>[2x]MTLSIPPSIQCQTEAACRLITRVTGDTLRAIHLYGSAVAGGLKPNSDIDLLVTICQPLTEAQRATLMQELLALSSPPGASAEKRALQVTVVLYSQLVPWCFPPSREMQFGEWLREDICQGIYEPAQQDWDMVLLITQILETSIPLKGERAERLFTPAPAAQLLKALRYPLDLWQSTADVQGDEYHIVLTLARIWYTLSTGRFTSKDAAADWLLPQLPEDYAATLRAAQREYLGLEQQDWHILLPAVVRFVDFAKAHIPTQFTKGHHHHHH

Aminoglycoside (3″)(9) adenylyltransferase AadA from Salmonella enterica belongs to the ANT(3″)-Ia family and catalyzes the magnesium-dependent O-adenylation of streptomycin and spectinomycin at positions 3″ and 9, respectively. Modification of streptomycin and spectinomycin by O-phosphorylation or O-nucleotidylation prevents the drugs from binding to their respective binding sites on the ribosome (for reviews, see Refs. 9 and 10). In the apo state, AadA has a monomeric two-domain structure with the active site located between an N-terminal adenylyltransferase domain and a C-terminal helical domain. We here present crystal structures of wild type (WT) AadA with ATP or ATP and streptomycin and of an active-site mutant in complex with ATP and streptomycin or dihydrostreptomycin.

The structure of AadA(E87Q) with ATP and streptomycin (AadA(E87Q)–ATP–sry) was refined to 1.73-Å resolution, and the structure of AadA(E87Q) with ATP and dihydrostreptomycin (AadA(E87Q)–ATP–dhs) was resolved to 1.4-Å resolution. Dihydrostreptomycin only differs from streptomycin in the reduction of the carbonyl group at the 3′-position, and because this position does not show any interaction with the protein and the two structures are virtually identical (r.m.s.d. of 0.2 Å over 261 Cα atoms), further analysis will be based on the dihydrostreptomycin structure. The overall structure of AadA(E87Q)–ATP–dhs is very similar to AadA–ATP (r.m.s.d. of 0.3 Å over 252 Cα atoms). Dihydrostreptomycin is bound between the two domains of AadA with the C ring sandwiched between the two domains in proximity of ATP, whereas the B- and A rings extend further toward the surface and form their major interactions with the C-terminal domain. AadA hides 417 Å2 (58%) of the van der Waals area of dihydrostreptomycin and makes interactions with all three rings. The C ring is the site of modification and is situated in proximity of the suggested catalytic base Glu-87 (mutated to glutamine in the structure) with the 3″-hydroxyl situated in the closest position. Furthermore, the ring is also oriented through a hydrogen bond of Asp-182 with the 6″-hydroxyl group and a stacking interaction with Trp-112. In turn, the B ring is oriented by His-185 through a hydrogen bond with the 3′-hydroxyl group. Finally, the A ring displays multiple interactions with the enzyme. Hydrogen bond interactions occur between Trp-173 and hydroxyl groups at positions 5 and 6, between the backbone carbonyl of Ala-177 and the guanidinium group at position 1, and between the backbone carbonyl of Asp-178 and the 6-hydroxyl group.> MKLERVTVKNFRSHSDTVVEFKEGINLIIGQNGSGKSSLLDAILVGLYWPLRIKDIKKDEFTKVGARDTYIDLIFEKDGTKYRITRRFL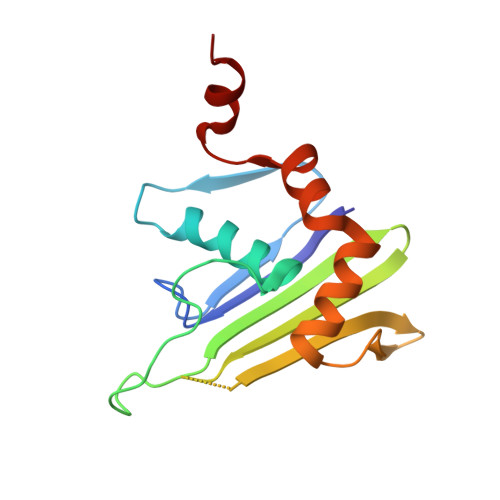KGYSSGEIHAMKRLVGNEWKHVTEPSSKAISAFMEKLIPYNIFLNAIYIRQGQIDAILES>[2x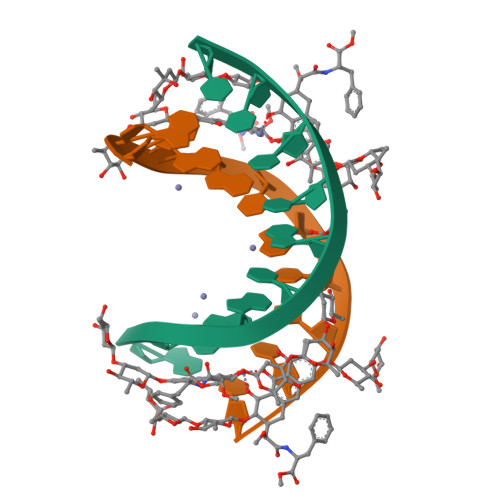]AGGGTACCCT>GSEDRDPTQFEERHLKFLQQLGKGNFGSVEMCRYDPLQDNTGEVVAVKKLQHSTEEHLRDFEREIEILKSLQHDNIVKYKGVCYSAGRRNLKLIMEY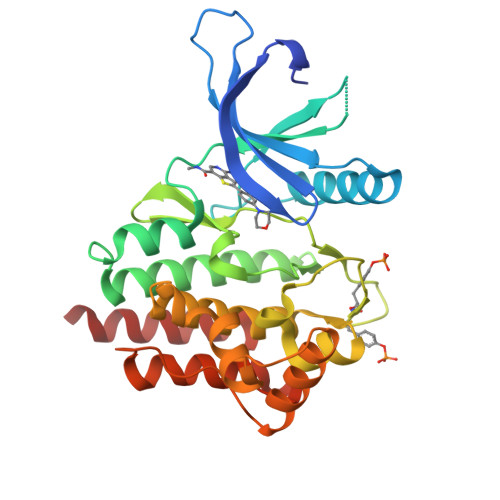LPYGSLRDYLQKHKERIDHIKLLQYTSQICKGMEYLGTKRYIHRDLATRNILVENENRVKIGDFGLTKVLPQDKEYYKVKEPGESPIFWYAPESLTESKFSVASDVWSFGVVLYELFTYIEKSKSPPAEFMRMIGNDKQGQMIVFHLIELLKNNGRLPRPDGCPDEIYMIMTECWNNNVNQRPSFRDLALRVDQIRDNMAG[2x]>SNAMLAEFEDRVAGIPCLIVVTYWE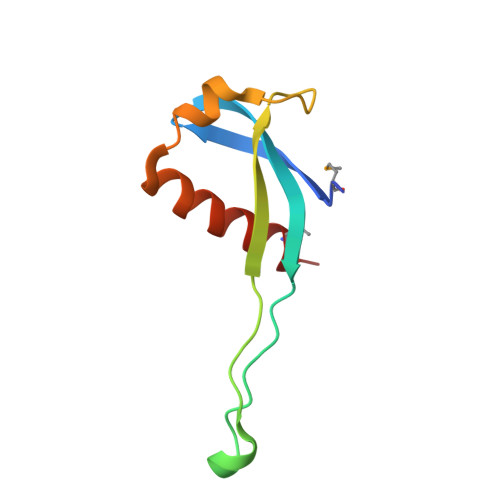PYVPAKVSGPPEYCYPAEGGCGEWEVRDRRGRPAPWLERKLTEAERERIDQAVFDRMEGR[2x]(1S,3S,4S,5R)-3-{4-amino-3-fluoro-5-[(1,1,1,3,3,3-hexafluoropropan-2-yl)oxy]benzyl}-5-[(3-tert-butylbenzyl)amino]tetrahydro-2H-thiopyran-4-ol 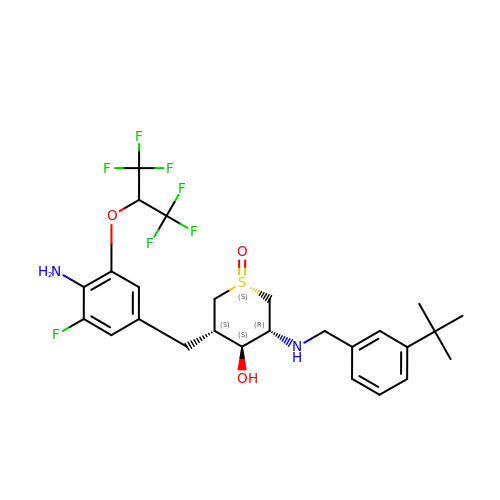1-oxide | C26 H31 F7 N2 O3 S | SVZBUJIOBQPGEC-DAMLKHMOSA-N> MKAQGETEDSERLSKMSSLLERLHAKFNQNRPWSETIKLVRQVMEKRVVMSSGGHQHLVSCLETLQKALKVTSLPAMTDRLESIARQNGLGSHLSASGTECYITSDMFYVEVQLDPAGQLCDVKVAHHGENPVSCPELVQQLREKNFEEFSKHLKGLVNLYNLPGDNKLKTKMYLALQSLEQDLSKMAIMYWKATNAAPLDKILHGSVGYLTPRSGGHLMNMKYYASPSDLLDDKTASPIILHEKNVPRSLGMNASVTIEGTSAMYKLPIAPLIMGSHPADNKWTPSFSAVTSANSVDLPACFFLKFPQPIPVSKAFVQKLQNCTGIPLFETPPTYLPLYELITQFELSKDPDPLPLNHNMRFYAALPGQQHCYFLNKDAPLPDGQSLQ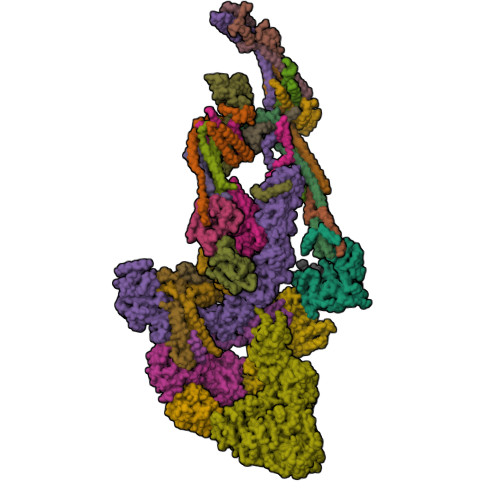GTLVSKITFQHPGRVPLILNMIRHQVAYNTLIGSCVKRTILKEDSPGLLQFEVCPLSESRFSVSFQHPVNDSLVCVVMDVQDSTHVSCKLYKGLSDALICTDDFIAKVVQRCMSIPVTMRAIRRKAETIQADTPALSLIAETVEDMVKKNLPPASSPGYGMTTGNNPMSGTTTPTNTFPGGPITTLFNMSMSIKDRHESVGHGEDFSKVSQNPILTSLLQITGNGGSTIGSSPTPPHHTPPPVSSMAGNTKNHPMLMNLLKDNPAQDFSTLYGSSPLERQNSSSGSPRMEMCSGSNKAKKKKSSRVPPDKPKHQTEDDFQRELFSMDVDSQNPMFDVSMTADALDTPHITPAPSQCSTPPATYPQPVSHPQPSIQRMVRLSSSDSIGPDVTDILSDIAEEASKLPSTSDDCPPIGTPVRDSSSSGHSQSALFDSDVFQTNNNENPYTDPADLIADAAGSPNSDSPTNHFFPDGVDFNPDLLNSQSQSGFGEEYFDESSQSGDNDDFKGFASQALNTLGMPMLGGDNGEPKFKGSSQADTVDFSIISVAGKALGAADLMEHHSGSQSPLLTTGELGKEKTQKRVKEGNGTGASSGSGPGSDSKPGKRSRTPSNDGKSKDKPPKRKKADTEGKSPSHSSSNRPFTPPTSTGGSKSPGSSGRSQTPPGVATPPIPKITIQIPKGTVMVGKPSSHSQYTSSGSVSSSGSKSHHSHSSSSSSLASASTSGKVKSSKSEGSSSSKLSGSMYASQGSSGSSQSKNSSQTGGKPGSSPITKHGLSSGSSSTKMKPQGKPSSLMNPSISKPNISPSHSRPPGGSDKLASPMKPVPGTPPSSKAKSPISSGSSGSHVSGTSSSSGMKSSSGSASSGSVSQKTPPASNSCTPSSSSFSSSGSSMSSSQNQHGSSKGKSPSRNKKPSLTAVIDKLKHGVVTSGPGGEDPIDSQMGASTNSSNHPMSSKHNTSGGEFQSKREKSDKDKSKVSASGGSVDSSKKTSESKNVGSTGVAKIIISKHDGGSPSIKAKVTLQKPGESGGDGLRPQIASSKNYGSPLISGSTPKHERGSPSHSKSPAYTPQNVDSESESGSSIAERSYQNSPSSEDGIRPLPEYSTEKHKKHKKEKKKVRDKDRDKKKSHSMKPENWSKSPISSDPTASVTNNPILSADRPSRLSPDFMIGEEDDDLMDVALIGN;> MAASSSGEKEKERMGGVSGMAGLGSTRERLLSALEDLEVLSRELIEMLAISRNQKLLQLEEENQVLELLIHRDGDFQELMKLALNQGKVHHEMQALEKEVEKRDSDIQQLQKQLKEAEQILATAVYQAKEKLKSIEKARKGAISSEEIIKYAHRISASNAVCAPLTWVPGDPRRPYPTDLEMRSGLLGQMNNPSTSGVNGHLPGDALAAGRLPDVLAPQYPWQSNDMSVNMLPPNHSSDFLLEPPGHNKENEDDVEVMSTDSSSSSSDSD;> MAAVDIRDNLLGISWVDSSWIPILNSGSVLDYFSERSNPFYDRTCNNEVVKMQRLTLEHLNQMVGIEYILLHAQEPILFIIRKQQRQSPAQVIPLADYYIIAGVIYQAPDLGSVINSRVLTAVHGIQSAFDEAMSYCRYHPSKGYWWHFKDHEEQEKVKPKAKRKEEPSSIFQRQRVDALLIDLRQKFPPRFVQQKSGEKPVPVDQAKKEAEPLPETVKSEEKESTKNIQQTVSTKGPPEKRMRLQ;> MGEPQQVSALPPPPMQYIKEYTDENIQEGLAPKPPPPIKDSYMMFGNQFQCDDLIIRPLESQGIERLHPMQFDHKKELRKLNMSILINFLDLLDILIRSPGSIKREEKLEDLKLLFVHVHHLINEYRPHQARETLRVMMEVQKRQRLETAERFQKHLERVIEMIQNCLASLPDDLPHSEAGMRVKAEPMDTDDNSNCPGQNEQQRESSGHRRDQIIEKDAALCVLIDEMNERP;> MQREEKQLEASLDALLNQVADLKNSLGSFIYKLENEYDRLTWPSVLDSFALLSGQLNTLNKVLKHEKTPLFRNQVIIPLVLSPDRDEDLMRQTEGRVPVFSHEVVPDHLRTKPDPEVEEQEKQLTTDAARIGADAAQKQIQSLNKMCSNLLEKISKEERESESGGLRPNKQTFNPGDTNALVAAVAFGKGLSNWRPSGSSGPGQPGQPGAGTILAGASGLPQVQMPGAPNQQQPMLSGVQMAQAGQPGKMPSGIKTNIKSASMHPYQR;> MASSGVAGGRQAEDTLQPPPELLPESKPPPPPQPLPVAALPPPAAPRPQSPAGAKEENYSFLPLVHNVIKCMDKDSPDLHQDLNALKTKFQELRKLIGTMPGIHVSPEQQQQQLHSLREQVRTKNELLQKYKSLCMFEIPKD;> MAEKFDHLEEHLEKFVENIRQLGIIVSDFQPSSQAGLSQKLNFIVTGLQDIDKCRQQLHDITVPLEVFEYIDQGRNPQLYTKECLERALAKNEQVKGKIDTMKKFKSLLIQELSKVFPEDMAKYRSIRGEDHPPS;> MATYSLANERLRALEDIEREIGAILQNAGTAILELSKEKTNERLLDRQAAAFTTSVQHVEAELSAQIRYLTQVATGQPHEGSSYSSRKDCQMALKRVDYARLKISDVARTCEQMLEN;> MAPVQLDNHQLIPPGGGGGSSGGGGSSSGSASAPAPPPPAAAVAAAAAAAASPGYRLSTLIEFLLHRAYSELMVLTDLLPRKSDVERKIEIVQFASRTRQLFVRLLALVKWANDAGKVEKCAMISSFLDQQAILFVDTADRLASLARDALVHARLPSFAIPYAIDVLTTGSYPRLPTCIRDKIIPPDPITKIEKQATLHQLNQILRHRLVTTDLPPQLANLTVANGRVKFRVEGEFEATLTVMGDDPEVPWRLLKLEILVEDKETGDGRALVHSMQIDFIHQLVQSRLFADEKPLQDMYNCLHCFCLSLQLEVLHSQTLMLIRERWGDLVQVERYHAGKSLSLSVWNQQVLGRKTGTASVHKVTIKIDENDVSKPLQIFHDPPLPASDSKLVERAMKIDHLSIEKLLIDSVHARAHQRLQELKAILRSFNANESSSIETALPALIVPILEPCGNSECLHIFVDLHSGMFQLMLYGLDPATLEDMEKSLNDDMKRIIPWIQQLKFWLGQQRCKQSIKHLPTITTETLQLANYSTHPIGSLSKNKLFIKLTRLPQYYIVVEMLEVPNKPTQLSYNYYFMSVSTADREDSPVMALLLQQFKDNIQDLMSYTKTGKQTRTGTKHKLSDDPCPIDSKKAKRSGEMCAFNKVLAHFVAMCDTNMPFVGLRLELSNLEIPHQGVQVEGDGFNHAIRLLKIPPCKGISEETQKALDRSLLDCTFRLQGRNNRTWVAELVFANCPLNGTSTREQGPSRHVYLTYENLLSEPVGGRKVVEMFLNDWSSIARLYECVLEFARSLPEIPAHLNIFSEVRVYNYRKLILCYGTTKGSSISIQWNSIHQKFHIALGTVGPNSGCSNCHNTILHQLQEMFNKTPNVVQLLQVLFDTQAPLNAINKLPTVPMLGLTQRTNTAYQCFSILPQSSTHIRLAFRNMYCIDIYCRSRGVVAIRDGAYSLFDNSKLVEGFYPAPGLKTFLNMFVDSNQDARRRSVNEDDNPPSPIGGDMMDSLISQLQPPQQQPFPKQPGTSGAYPLTSPPTSYHSTVNQSPSMMHTQSPGNLHAASSPSGALRAPSPASFVPTPPPSSHGISIGPGASFASPHGTLDPSSPYTMVSPSGRAGNWPGSPQVSGPSPATRLPGMSPANPSLHSPVPDVSHSPRAGTSSQTMPTNMPPPRKLPQRSWAASIPTILTHSALNILLLPSPTPGLVPGLAGSYLCSPLERFLGSVIMRRHLQRIIQQETLQLINSNEPGVIMFKTDALKCRVALSPKTNQTLQLKVTPENAGQWKPDELQVLEKFFETRVAGPPFKANTLIAFTKLLGAPTHILRDCVHIMKLELFPDQATQLKWNVQFCLTIPPSAPPIAPPGTPAVVLKSKMLFFLQLTQKTSVPPQEPVSIIVPIIYDMASGTTQQADIPRQQNSSVAAPMMVSNILKRFAEMNPPRQGECTIFAAVRDLMANLTLPPGGRP;> MDVSGQETDWRSAAFRQKLVSQIEDAMRKAGVAHSKSSKDMESHVFLKAKTRDEYLSLVARLIIHFRDIHNKKSQASVSDPMNALQSLTGGPTPGAAGIGMPPRGPGQSLGGMGGLGAMGQPLPLSGQPPPGTSGMAPHGMAVVSTATPQTQLQLQQVALQQQQQQQQQQQFQQQQAALQQQQQQQQQQQQQQQFQAQQNAMQQQFQAVVQQQQLQQQQQQQHLIKLHHQSQQQQIQQQQLQRMAQLQLQQQQQQQQQQALQAQPPMQQPSMQQPQPPPSQALPQQLSQLHHPQHHQPPPQAQQSPIAQNQPPQIPPQSQSQPLVSQAQALPGPMLYAAQQQLKFVRAPMVVQQPQVQPQVQQVQPQVQPQAAVQAAQSAQMVAPGVQMIAEALAQGGMHVRARFPPTSTMSAGPSSSISLGGQPTTQVSQSSLTMLSSPSPGQQVQTPQSMPPPPQPSPQPGSQPNSNVSSGPAPSPSSFLPSPSPQPSQSPVTARTPQNFSVPSPGPLNTPVNPSSVMSPAGSSQAEEQQYLDKLKQLSKYIEPLRRMINKIDKNEDRKKDLSKMKSLLDILTDPSKRCPLKTLQKCEIALEKLKNDMAVPTPPPPPVLPTKQQDLCQPLLDAVLANIRSPVFNHSLYRTFVPAMMAIHGPPIVSPVVCSRKRRFEEDERQSIPNVLQGEVARLDPKFLVNLDPSHCSNNGTVHLICKLDDKDLPSVPPLELSVPADYPAQSPMWIDRQWQYDANPFLQSVHRCMTSRLLQLPDKHSVTALLNTWAQSIHQACLSAA;> MDLAYVCEWEKWAKSTYCPSLPLACAWSCRNLIAFTTDLRNDDQDLTHMIHILDTEHPWEVHSVSSGHSEAITCLEWDQSGSRLLSADADGQIKCWSMADHLANSWESSVGSQVEGDPIVALSWLHNGVKLALHVEKSGASSFGEKFSRVKFSPSLTLFGGKPMEGWIAVTVSGLVTVSLLKPSGQVLTSTESLCRLRGRVALADIAFTGGGNIVVAAADGSSASPVKFYKVCVSVVSEKCRIDTEILPSLFMRCTTDPNRKDRFPAITHLKFLARDMSEQVLLCASSQTSSLVECWSLRKEGLPVNNIFQQISPVVGDKQPMILKWRILSATNDLDRVSAVALPKLPISLTNTDLKVASDTQFYPGLGLALAFQDGSVHMVHRLSLQTMAVFYSSAPRSLDEPALKRPRTTCPAVHFKAMQLSWTSLALVGIDNHGKLSMLRISPSLGHPLEPKLALQHLLFLLEYCMVTGYDWWDILLHVQPGMVQSLVERLHEEYTRQKPALQQVLSTRILAMKASLCKLSPCTVARVCDYHTKLFLMAITSTLKSLLRPHFLNTPDKSPGDRLAEICAKITDVDIDKVMINLKTEEFVLDMNTLQALQQLLQWVGDFVLYLLVSLPNQGSPLRPGHSFLRDGTSLGMLRELMVVIRIWGLLKPSCLPVYTATSDTQDSMSLLFRLLTKLWICCRDEGAASEPDEGLVDECCLLPSQLLVPNLDWLPASDGLVSRLQPKQPLRLRFGRAPTLPSSTSTLQLDGLTRAPGQPKIDHLRRLHLGAYPTEECKACTRCGCVTMLKSPNKTTAVTQWEQRWIKNCLCGGLWRRVPLSCS;> MSGVRAVRISIESACEKQVQEVGLDGTETYLQPLSMSQNLARLAQRIDFSQGSGSEEEEAAGPDGDAPDWGGAGADQDDEEGLVKFQPSLWPWDSVRNNLRSALTEMCVLYDVLSIVRDKKFMTLDPVSQDALPPKQSPQTLQLISKKKSLAGAAQILLKGAERLTKSVAENQENKLQRDFNSELLRLRQHWKLRKVGDKILGDLSYRSAGSLFPHHGTFEVIKNTDIDLDKKIPEDYCPLDVQIPSDLEGSAYIKVSIQKQAPDIGDLGTVNLFKRPLPKSKPGSPHWQTKLEAAQNVLLCKEIFAQLSREAVQIKSQIPHIVVKNQIISQPFPSLQLSISLCHSSDDKKSQKCAAEKPGQEDHLYVLEHNLHLLIREFHKQTLSSIVMPHPASAPFGHKRMRLSGPQAFDKNEINSIQSTEGLLEKIIKQAKHIFLRSRTAATIDSLASRIEDPQIQAHWSNINDVYESSVKVLITSQGYEQICKSIQLQLNIGVEQVRVVHRDGRVIMLSHQEQELQDFLLSQMSQHQVHAVQQLAKVMGWQVLSFSNHVGLGPIESIGNASAITVASPSGDYAISVRNGPESGSKIMVQFPRNQCKDLPKSDVLQDSKWSHLRGPFKEVQWNKMEGRNFVYKMELLMSALSPCLL;> MEAPPVTMMPVTGGTINMMEYLLQGSVLDHSLESLIHRLRGLCDNMEPETFLDHEMVFLLKGQQASPFVLRARRSMDRAGAPWHLRYLGQPEMGDKNRHALVRNCVDIATSENLTDFLMEMGFRMDHEFVAKGHLFRKGIMKVVVYKIFRILVPGNTDSTEALSLSYLVELSVVAPAGQDMVSDDMRNFAEQLKPLVHLEKIDPKRLM;> MENFTALFGAQTDPPPPPSALGFGPGKPPPPPPPPPGGGPGAAPPSTATSAPAGADKSTAGSGPFYLMRELPGSTELTGSTNLITHYNLEQAYNKFCGKKVKEKLSNFLPDLPGMIDLPGSHDNSSLRSLIEKPPILGGSFNPITGTMLSGFRLHTGPLPEQCRLMHIQPPKKKNKHKHKQSRTQDPVPPETPSDSDHKKKKKKKEEDPERKRKKKEKKKKKNRHSPDHPGMGSSQASSS;> MGVTCVSQMPVAEGKSLQQTVELLTKKLEMLGAEKQGTFCVDCETYHTAASTLGSQGQAGKLMYVMHNSEYPLSCFALFENGPCLIADTNFDVLMVKLKGFFQSAKASKIETRGTRYQYCDFLVKVGTVTMGPSARGISVEVEYGPCVVASDCWSLLLEFLQSFLGSHAPGAPTVFGNRHDAVYGPADTMIQYMELFNKIRKQQQVPVAGIR;> MADRLTQLQDAVNSLADQFCNAIGVLQQCGPPASFSNIQTAINKDQPANPTEEYAQLFAALIARTAKDIDVLIDSLPSEESTAALQAASLYKLEEENHEAATCLEDVVYRGDMLLEKIQSALADIAQSQLKTRSVTHSHSLPDS;> MAQQRALPQSKETLLQSYNKRLKDDIKSIMDNFTEIIKTAKIEDETQVSRATQGEQDNYEMHVRAANIVRAGESLMKLVSDLKQFLILNDFPSVNEAIDQRNQQLRALQEECDRKLITLRDEVSIDLYELEEEYYSSSSSLCEANDLPLCEAYWRLDLDADSADGLSAPLLASPETGAGPLQSAAPVHSHGGGPGPTEHT;> METQLQSIFEEVVKTEIIEEAFPGMFMDTPEDEKTKLISCLAAFRQFWSGLSQESHEQCVQWIVKFIHGQHSPKRISFLYDCLAMAVETGLLPPRMVCESLINSDSLEWERTQLWALTFKLVRKIIGGVDYKGVRDLLKAILEKILTIPNTVSSAVVQQLLAAREVIAYILERNACLLPAYFAVTEIRKLYPEGKLPHWLLGNLVSDFVDTFRPTARINSICGRCSLLPVVNNSGAICNSWKLDPATLRFPLKGLLPYDKDLFEPQTALLRYVLEQPYSRDMVCNMLGLNKQHKQRCPVLEDQLVDLVVYAMERSETEEKFDDGGTSQLLWQHLSSQLIFFVLFQFASFPHMVLSLHQKLAGRGLIKGRDHLMWVLLQFISGSIQKNALADFLPVMKLFDLLYPEKECIPVPDINKPQSTHAFAMTCIWIHLNRKAQNGDSTLQIPIPHSLKLHHEFLQQSLRNKSLQMNDYKIALLCNAYSTNSECFTLPMGALVETIYGNGIMRVPLPGTSCLASASVTPLPMNLLDSLTVHAKMSLIHSIATRVIKLAHTKSSVALAPALVETYSRLLVYMEIESLGIKGFISQLLPTVFKSHAWGILHTLLEMFSHRMHHIQPHYRVQLLSHLHTLAAVAQTNQNQLHLCVESTALRLITALGSSEVQPQFTRFLNDPKTVLSAESEELNRALILTLARATHVTDFFTGSDSIQGTWCKDILQTIMNFTPHNWASHTLSCFPAPLQAFFKQNNVPQESRFNLKKNVEEEYRKWKSMTDENEIITQFSVQGFPPLFLCLLWKMLLETDHISQIGYKVLERIGARALVAHVRTFADFLVYEFSTSAGGQQLNKCIEILNDMVWKYNIVTLDRLILCLAMRSHEGNEAQVCYFIIQLLLLKPNDFRNRVSDFVKENSPEHWLQSDWHTKHMSYHKKYPEKLYFEGLAEQVDPPVPIQSPYLPIYFGNVCLRFLPVFDIVIHRFLELLPVSKSLETLLDHLGGLYKFHDRPVTYLYNTLHYYEMCLRNRDHLKRKLVHAIIGSLKDNRPQGWCLSDTYLKHAMNAREDNPWVPEDSYYCKLIGRLVDTMAGKSPGPFPNCDWRFNEFPNPAAHALHVTCVELMALAVPGKDVGNALLNVVLKSQPLVPRENITAWMNAIGLIITALPEPYWIVLHDRIVNVISSSSLTSETEWVGYPFRLFDFTACHQSYSEMSCSYTLALAHAVWHHSSIGQLSLIPKFLTEALLPVVKTEFQLLYVYHLVGPFLQRFQQERTRCMIEIGVAFYDMLLNVDQCSTHLNYMDPICDFLYHMKYMFTGDSVKEQVEKIICNLKPALKLRLRFITHISKMEPAVPPQALNSGSPAPQSNQVPASLPVTQ;> MKVVNLKQAILQAWKERWSDYQWAINMKKFFPKGATWDILNLAEALLEQAMIGPSPNPLILSYLKYAISSQMVSCSSVLTAISKFDDFSRDLCVQALLDIMDMFCDRLSCHGKAEECIGLCRALLSALHWLLRCTAASAERLQEGLEAGTPAPGEKQLALCLQCLEKTLSSTKNRALLHIAKLEEASSWTAIEHSLLKLGEILANLSNPQLRSQAERCGTLIRSIPSMLSVHSEQLHKTGFPTIHALILLEGTMNLTGEMQPLVEQLMMVKRMQHIPTPLFVLEIWKACFVGLIESPEGTQELKWTAFTYLKIPQVLVKLKKYFHGEKDFTEDVNCAFEFLLKLTPLLDKADQRCNCDCTNFLLQECNKQGLLSEVNFASLVGKRTADRDPQLKSSENANIQPNPGLILRAEPTVTNILKTMDADHSKSPEGLLGVLGHMLSGKSLDLLLAAAAATGKLKSFARKFINLNEFTTHGSGESTKTASVRALLFDISFLMLCHVAQTYGSEVILSESSSGEEVPFFETWMQTCMPEEGKILNPDHPCFRPDSTKVESLVALLNNSSEMKLVQMKWHEACLSISAAILEILNAWENGVLAFESIQKITDNIKGKVCSLAVCAVAWLVAHVRMLGLDEREKSLQMIRQLAGPLYSENTLQFYNERVVIMNSILEHMCADVLQQTATQIKFPSTGVDTMPYWNLLPPKRPIKEVLTDIFAKVLEKGWVDSRSIHILDTLLHMGGVYWFCNNLIKELLKETRKEHTLRAVQLLYSIFCLDMQQVTLVLLGHILPGLLTDSSKWHSLMDPPGTALAKLAVWCALSSYSSHKGQASSRQKKRHREDIEDYVSLFPVEDMQPSKLMRLLSSSDDDANILSSPTDRSMNSSLSASQLHTVNMRDPLNRVLANLFLLISSILGSRTAGPHTQFVQWFMEECVGCLEQDSRGSILQFMPFTTVSELVKVSAMSSPKVVLAITDLSLPLGRQVAAKAIAAL;> MVPGSEGPARAGGLVADVVFVIEGTANLGPYFEELRKHYLLPAIEYFNGGPPAETDFGGDYGGTQYSLVVFNTVDCAPESYVQCHAPTSSAYEFVTWLDGIKFMGGGGESCSLIAEGLSTALQLFDDFKKMREQIGQTHRVCLLICNSPPYLLPAVESTTYSGCTTESLVQKIGERGIHFSIVSPRKLPALRLLFEKAAPPALLEPLQQPADVSQDPRHMVLVRGLVLPVGGSSTSGSLQTKQAVPLPPAPASAATLSAAPPQALPPVPPQYQVPGNLSAAQVAAQNAVEAAKSQKAGLGPRFSPINPLQQAAPGVGPPFSQAPAPPLAPVPPGAPKPPPASQPSLVSTVAPGPVLAAPAQPGAPSLAGTVTPGGVNGPSAAQLGGPALGGQQSVSNKLLAWSGVLEWQEKPKPASVDANTKLTRSLPCQVYVNHGENLKTEQWPQKLIMQLIPQQLLTTLGPLFRNSRMVQFHFTNKDLESLKGLYRIMGNGFAGCVHFPHTAPCEVRVLMLLYSSKKKIFMGLIPYDQSGFVNGIRQVITNHKQVQQQKLEQQRGMGAQQAPPVLGPILEEQARPPQNLLQLRAPQPQPQGAVGASAATGQPQPQGATQAPTGAPQGPPGAAPGPPPSGPILRPQNPGANPQLRSLLLNPAPPQTGVPPPQASLHHLQPPGAPTLLPPHQSMGQPQLGPQLLHPPPAQSWPTQLPQRAPLPGQMLLSGGPRGPVPQPGLQPSVMEDDILMDLI;> MTAAPASPQQMRDRLLQAIDSQSNIRNMVAVLEVISSLERYPITKEALEETRLGKLINDVRKKTKNEELAKRAKRLLRSWQKLIEPVHQNEVALRALAGAAGSANGGAHNCRPEMGVAGAPKSIHDLKNRNDIQRLPGQRLDRLGSRKRRGDQRDLGHPGPPHKVSKGSPDPLVPNASPLPTNGISGSPESLPSPLDGSGHLGPDGSRLEPSDNEKHSTKIPVNAVRPRPSSPGLGKPPVPCLQTKAAQLQQLDRADESPGPPYPRGSSRCSFSPRNSRHEGSFSRHRSSYIPKGQVSSPSPWPQPPDNTQVPSPLPLAQPPTPPVRRQELLPNAESPVHWPEQSEGHPRLTGPACRAGFSPDSSKADSDATSSGGSDSKKKKRYRPRDYTVNLDGQVAEAGVKPVRLKERKLTFDPMTRQIRPLTQKEPVRADSPVPTEQLPRTELEQQEVKASLQSPFEQTNWKELSRNEIIQSYLSRQSSLLSSSGAQTPGAHHFMAEYLKQEESSRQGARQPHVLLPLPTPTDLPGLTREVTQDDLDRIQAQQWPGVNGCEDTQGNWYDWTQCISLDPHGDDGRLNILPYVCLD;> MADVLSVGVNLEAFSQAISAIQALRSSVSRVFDCLKDGMRNKETLEGREKAFIANFQDNLHSVNRDLNELERLSNLVGKPSENHPLHNSGLLSLDPVQDKTPLYSQLLQAYKWSNKLQYHAGLASGLLNQQSLKRSANQMGVSAKRRPKAQPTTLVLPPQYVDDVISRIDRMFPEMSIHLSRPNGTSAMLLVTLGKVLKVIVVMRSLFIDRTIVKGYNESVYTEDGKLDIWSKSSYQVFQKVTDHATTALLHYQLPQMPDVVVRSFMTWLRSYIKLFQAPCQRCGKFLQDGLPPTWRDFRTLEAFHDTCRQ;> MAASLGGMFTGQPPGPPPPPPGLPGQASLLQAAPGAPRPSNSTLVDELESSFEACFASLVSQDYVNGTDQEEIRTGVDQCIQKFLDIARQTECFFLQKRLQLSVQKPDQVIKEDVSELRSELQRKDALVQKHLTKLRHWQQVLEDINVQHKKPADMPQGSLAFLEQASANIPAPLKQT;> MAAPQPQAAAVSSASGVSGPGSAGGPGPQQQPQPTQLVGSAQSGLLQQQQQDFDPVQRYKMLIPQLKESLQTLMKVAAQNLIQNTNIDNGQKSSDAPLQRFDKCLEEFYALCDQLELCLRLAHECLSQSCDSAKHSPTLVPTATKPDAVQPDSLPYPQYLAVIKAQITCAKDIHTALLDCANKVTGKTTAPSTGPGGSL;> MSTPPLAPTGMASGPFGGPQAQQAAREVNTATLCRIGQETVQDIVYRTMEIFQLLRNMQLPNGVTYHTGTYQDRLTKLQDHLRQLSILFRKLRLVYDKCNENCGGMDPIPVEQLIPYVDEDGSKNDDRAGPPRFASEERREIVEVNKKLKQKNQQLKQIMDQLRNLIWDINAMLAMRN;> MAAAVAMETDDAGNRLRFQLELEFVQCLANPNYLNFLAQRGYFKDKAFVNYLKYLLYWKEPEYAKYLKYPQCLHMLELLQYEHFRKELVNAQCAKFIDEQQILHWQHYSRKRVRLQQALAEQQQQNNTAGK Kynurenine 3-monooxygenase (KMO) regulates levels of neuroactive kynurenine pathway metabolites associated with neurodegeneration. Downregulation of KMO activity shifts the flux between the two branches of the KP toward increased KYNA formation, thus generating a neuroprotective environment. The KMO reaction is a random bi–bi mechanism proceeding through a ternary complex of KMO-bound to l-KYN and NADPH (steady-state enzymatic assays are described in Supplementary Methods) with a turnover value, kcat, of 8.2 ± 0.2 s−1 and Km values for NADPH and l-KYN of 16.9 ± 1.5 and 12.1 ± 1.4 µM, respectively. We next determined crystal structures of KMO in complex with the novel inhibitors or with l-KYN to inform the design of small-molecule inhibitors capable of penetrating the blood–brain barrier.

Compounds 9, 11–13 and 16–19 are structurally similar to the KMO inhibitor 6-(3,4-dichlorophenyl) pyrimidine-4-carboxylic acid, in which the pyrimidine ring of the reported inhibitor is replaced by an isosteric furan ring in 9, 11–13 and 16–19. To validate binding modes of the four inhibitors for which crystal structures were obtained (1, 4, 9 and 13), we investigated their mechanisms of inhibition. Consistent with the crystal structures, each compound was found to be a competitive inhibitor of l-KYN. Inhibitor 9 is also a competitive inhibitor of NADPH, whereas compounds 1, 4 and 13 were mixed type inhibitors with respect to NADPH. In each case, the inhibitor was bound in the l-KYN-binding pocket, with the chlorinated aromatic moiety occupying a similar position to the substrate l-KYN aniline group. Furthermore, the carboxylate group of the inhibitor was in close proximity to PfKMO R83/Y97/N368. Notably, inhibitors 1, 4, 9, 13 do not stimulate KMO reduction by NADPH in rapid mixing stopped-flow assays. H2O2 production was not detected with compound 1 and PfKMO using a coupling reaction with o-dianisidine and horseradish peroxidase in the presence and absence of l-Kyn. This suggests that 1, 4, 9, 13 inhibit KMO activity in the absence of H2O2 production and thus may be preferable for therapeutic application.

>TATDNARQVTIIGAGLAGTLVARLLARNGWQVNLFERRPDPRIETGARGRSINLALAERGAHALRLAGLEREVLAEAVMMRGRMVHVPGTPPNLQPYGRDDSEVIWSINRDRLNRILLDGAEAAGASIHFNLGLDSVDFARQRLTLSNVSGERLEKRFHLLIGADGCNSAVRQAMASVVDLGEHLETQPHGYKELQITPEASAQFNLEPNALHIWPHGDYMCIALPNLDRSFTVTLFLHHQSPAAQPASPSFAQLVDGHAARRFFQRQFPDLSPMLDSLEQDFEHHPTGKLATLRLTTWHVGGQAVLLGDAAHPMVPFHGQGMNCALEDAVALAEHLQSAADNASALAAFTAQRQPDALAIQAMALENYVEMSSKVASPTYLLERELGQIMAQRQPTRFIPRYSMVTFSRLPYAQAMARGQIQEQLLKFAVANHSDLTSINLDAVEHEVTRCLPPLSHLS[2x]>[2x]ALFGSNDVTTAHSDYEIVLEGGSSSWGKVKARAKVNAPPASPLLPADCDVKLNVKPLDPAKGFVRISAVFESIVDSTKNKLTIEADIANETKERRISVGEGMVSVGDFSHTFSFEGSVVNLFYYRSDAVRRNVPNPIYMQGRQFHDILMKVPLDNNDLIDTWEGTVKAIGSTGAFNDWIRDFWFIGPAFTALNEGGQRISRIEVNGLNTES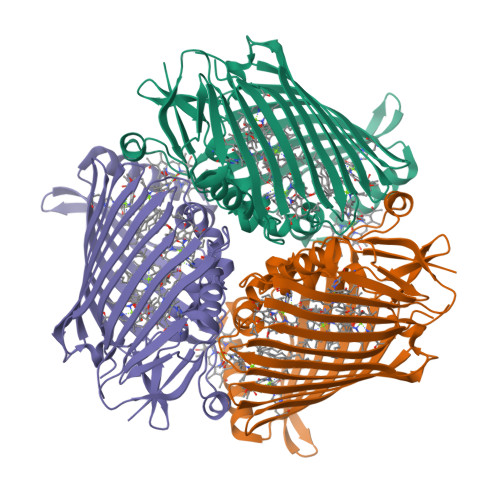GPKGPVGVSRWRFSHGGSGMVDSISRWAELFPSDKLNRPAQVEAGFRSDSQGIEVKVDGEFPGVSVDAGGGLRRILNHPLIPLVHHGMVGKFNNFNVDAQLKVVLPKGYKIRYAAPQYRSQNLEEYRWSGGAYARWVEHVCKGGVGQFEILYAQ>MKLSGGVEWALHCCVVLTAASRPVPAARLAELADVSPSYLAKQMQALSRAGLVRSVQGKTGGYVLTRPAVEITLLDVVQAVDGPDPAFVCTEIRQRGPLATPPEKCTKACPIARAM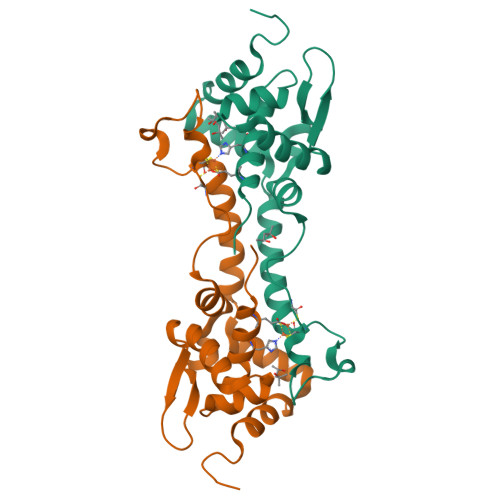GAAEAAWRASLAATTIADLVATVDDESGPDALPGVGAWLIEGLGHHHHHH[4x]>[8x]MTGMSREEVESLIQEVLEVYPEKARKDRNKHLAVNDPAVTQSKKCIISNKKSQPGLMTIRGCAYAGSKGVVWGPIKDMIHISHGPVGCGQYSRAGRRNYYIGTTGVNAFVTMNFTSDFQEKDIVFGGDKKLAKLIDEVETLFPLNKGISVQSECPIGLIGDDIESVSKVKGAELSKTIVPVRCEGFRGVSQSLGHHIANDAVRDWVLGKRDEDTTFASTPYDVAIIGDYNIGGDAWSSRILLEEMGLRCVAQWSGDGSISEIELTPKVKLNLVHCYRSMNYISRHMEEKYGIPWMEYNFFGPTKTIESLRAIAAKFDESIQKKCEEVIAKYKPEWEAVVAKYRPRLEGKRVMLYIGGLRPRHVIGAYEDLGMEVVGTGYEFAHNDDYDRTMKEMGDSTLLYDDVTGYEFEEFVKRIKPDLIGSGIKEKF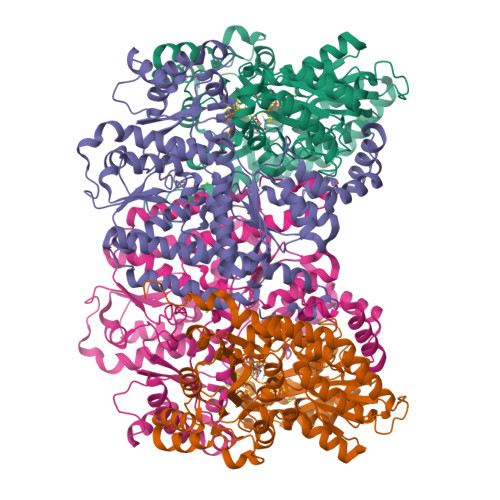IFQKMGIPFREMHSWDYSGPYHGFDGFAIFARDMDMTLNNPCWKKLQAPWE;>MSQQVDKIKASYPLFLDQDYKDMLAKKRDGFEEKYPQDKIDEVFQWTTTKEYQELNFQREALTVNPAKACQPLGAVLCALGFEKTMPYVHGSQGCVAYFRSYFNRHFREPVSCVSDSMTEDAAVFGGQQNMKDGLQNCKATYKPDMIAVSTTCMAEVIGDDLNAFINNSKKEGFIPDEFPVPFAHTPSFVGSHVTGWDNMFEGIARYFTLKSMDDKVVGSNKKINIVPGFETYLGNFRVIKRMLSEMGVGYSLLSDPEEVLDTPADGQFRMYAGGTTQEEMKDAPNALNTVLLQPWHLEKTKKFVEGTWKHEVPKLNIPMGLDWTDEFLMKVSEISGQPIPASLTKERGRLVDMMTDSHTWLHGKRFALWGDPDFVMGLVKFLLELGCEPVHILCHNGNERWKKAVDAILAASPYGKNATVYIGKDLWHLRSLVFTDKPDFMIGNSYGKFIQRDTLHKGKEFEVPLIRIGFPIFDRHHLHRSTTLGYEGAMQILTTLVNSILERLDEETRGMQATDYNHDLVR[8x]>[2x]MALLAEHLLKPLPADKQIETGPFLEAVSHLPPFFDCLGSPVFTPIKADISGNITKIKAVYDTNPAKFRTLQNILEVEKEMYGAE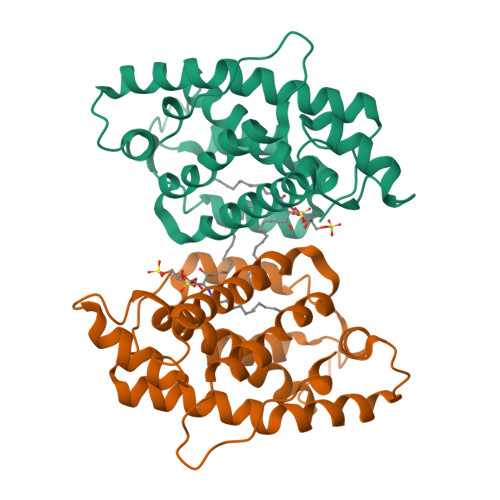WPKVGATLALMWLKRGLRFIQVFLQSICDGERDENHPNLIRVNATKAYEMALKKYHGWIVQKIFQAALYAAPYKSDFLKALSKGQNVTEEECLEKIRLFLVNYTATIDVIYEMYTQMNAELNYKV> QENRLLNESESSSQGLLGYYFSDLNFQAPMVVTSSTTGDLSIPSSELENIPSENQYFQSAIWSGFIKVKKSDEYTFATSADNHVTMWVDDQEVINKASN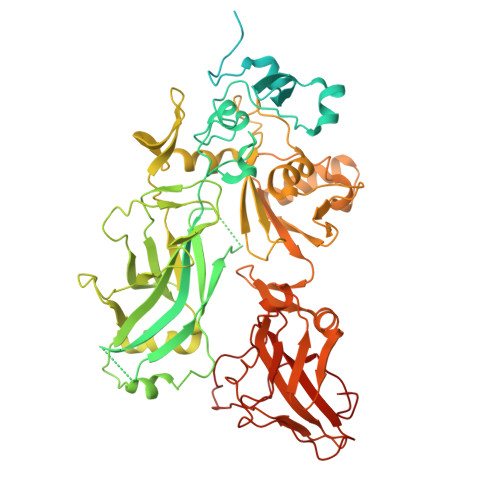SNKIRLEKGRLYQIKIQYQRENPTEKGLDFKLYWTDSQNKKEVISSDNLQLPELKQKSSNSLEVLFQGSTSAGPTVPDRDNDGIPDSLEVEGYTVDVKNKRTFLSPWISNIHEKKGLTKYKSSPEKWSTASDPYSDFEKVTGRIDKNVSPEARHPLVAAYPIVHVDMENIILSKNEDQSTQNTDSQTRTISKNTSTSRTHTSEVHGNAEVHASFFDIGGSVSAGFSNSNSSTVAIDHSLSLAGERTWAETMGLNTADTARLNANIRYVNTGTAPIYNVLPTTSLVLGKNQTLATIKAKENQLSQILAPNNYYPSKNLAPIALNAQDDFSSTPITMNYNQFLELEKTKQLRLDTDQVYGNIATYNFENGRVRVDTGSNWSEVLPQIQETTARIIFNGKDLNLVERRIAAVNPSKPLETTKPDMTLKEALKIAFGFNEPNGNLQYQGKDITEFDFNFDQQTSQNIKNQLAELNATNIYTVLDKIKLNAKMNILIRDKRFHYDRNNIAVGADESVVKEAHREVINSSTEGLLLNIDKDIRKILSGYIVEIEDTEGLKEVINDRYDMLNISSLRQDGKTFIDFKKYNDKLPLYISNPNYKVNVYAVTKENTIINPSENGDTSTNGIKKILIFSKKGYEIG>[3x]MNTISILSTTDLPAAWQIEQRAHAFPWSEKTFFGNQGERYLNLKLTADDRMAAFAITQVVLDEATLFNIAVDPDFQRRGLGRMLLEHLIDELETRGVVT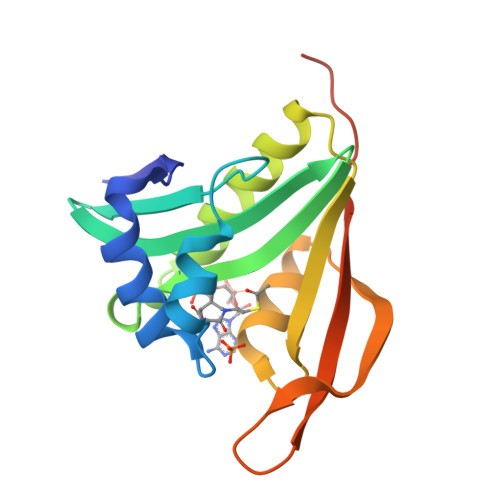LWLEVRASNAAAIALYESLGFNEATIRRNYYPTAQGHEDAIIMALPISMKLHHHHHHHHHH> GAMGYKDNIRHGVCWIYYPDGGSLVGEVNEDGEMTGEKIAYVYPDERTALYGKFIDGEMIEGKLATLMSTEEGRPHFELMPGNSVYHFDKSTSSCISTNALLPDPYESERVYVAESLISSAGEGLFSKVAVGPNTVMSFYNGVRITHQEVDSRDWALNGNTLSLDEETVIDVPEPYNHVSKYCASLGHKANHSFTPNCIYDMFVHPRFGPIKCIRTLRAVEADEELTV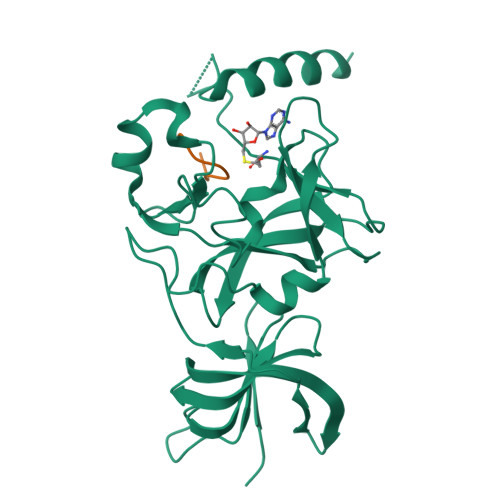AYGYDHSPPGKSGPEAPEWYQVELKAFQATQQK;> XSKSKDRKYTL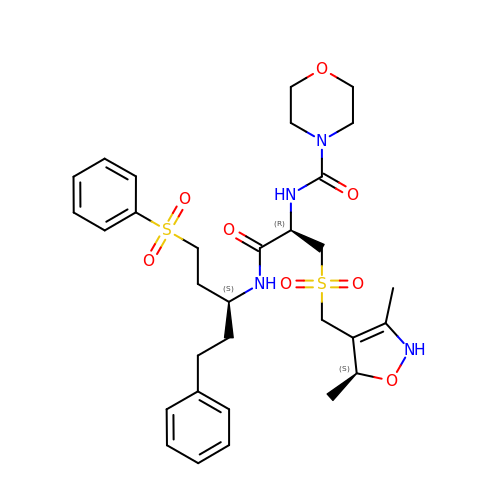N-[(1R)-1-[({[(5S)-3,5-DIMETHYL-2,5-DIHYDROISOXAZOL-4-YL]METHYL}SULFONYL)METHYL]-2-OXO-2-({(1S)-3-PHENYL-1-[2-(PHENYLSULFONYL)ETHYL]PROPYL}AMINO)ETHYL]MORPHOLINE-4-CARBOXAMIDE | C31 H42 N4 O8 S2 | KPLOSZKQTFPNFM-MIUCGUHXSA-N>[4x]ADKLPYKVADIGLAAWGRKALDIAENEMPGLMRMREMYSASKPLKGARIAGCLHMTVETAVLIETLVALGAEVRWSSCNIFSTQDHAAAAIAKAGIPVFAWKGETDEEYLWCIEQTLHFKDGPLNMILDDGGDLTNLIHTKHPQLLSGIRGISEETTTGVHNLYKMMANGILKV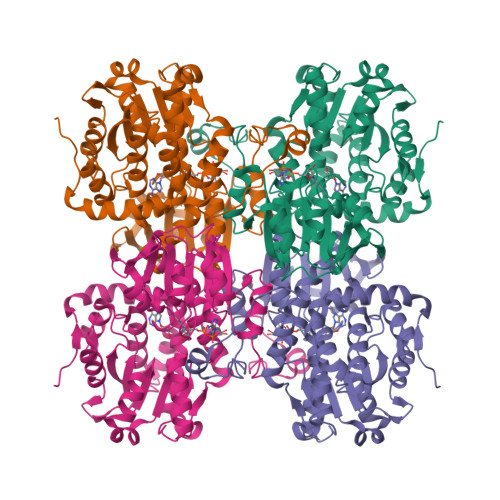PAINVNDSVTNSKFDNLYGCRESLIDGIKRATDVMIAGKVAVVAGYGDVGKGCAQALRGFGARVIITEIDPINALQAAMEGYEVTTMDEACKEGNIFVTTTGCVDIILGRHFEQMKDDAIVCNIGHFDVEIDVKWLNENAVEKVNIKPQVDRYLLKNGHRIILLAEGRLVNLGCAMGHPSFVMSNSFTNQVMAQIELWTHPDKYPVGVHFLPKKLDEAVAEAHLGKLNVKLTKLTEKQAQYLGMPINGPFKPDHYRY> MPKLVTWMNNQRVGELTKLANGAHTFKYAPEWLASRYARPLSLSLPLQRGNITSDAVFNFFDNLLPDSPIVRDRIVKRYHAKSRQPFDLLSEIGRDSVGAVTLIPEDETVTHPIMAWEKLTEARLEEVLTAYKADIPLGMIREENDFRISVAGAQEKTALLRIGNDWCIPKGITPTTHIIKLPIGEIRQPNATLDLSQSVDNEYYCLLLAKELGLNVPDAEIIKAGNVRALAVERFDRRWNARRTVLLRLPQEDMCQTFGLPSSVKYESDGGPGIARIMAFLMGSSEALKDRYDFMKFQVFQWLIGATQGHAKNFSVFIQAGGSYRLTPFYDIISAFPVLGGTGI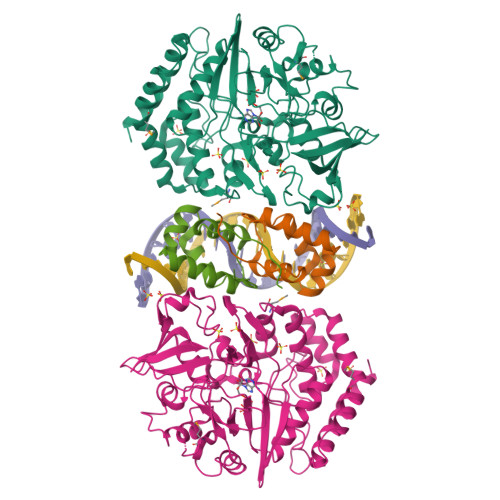HISDLKLAMGLNASKGKKTAIDKIYPRHFLATAKVLRFPEVQMHEILSDFARMIPAALDNVKTSLPTDFPENVVTAVESNVLRLHGRLSREYGSK;> MMSFQKIYSPTQLANAMKLVRQQNGWTQSELAKKIGIKQATISNFENNPDNTTLTTFFKILQSLELSMTLCDAKNASPESTEQQNLEW>MCGIWALFGSDDCLSVQCLSAMKIAHRGPDAFRFENVNGYTNCCFGFHRLAVVDPLFGMQPIRVKKYPYLWLCYNGEIYNHKKMQQHFEFEYQTKVDGEIILHLYDKGGIEQTICMLDGVFAFVLLDTANKKVFLGRDTYGVRPLFKAMTEDGFLAVCSEAKGLVTLKHSATPFLKVEPFLPGHYEVLDLKPNGKVASVEMVKYHHCRDVPLHALYDNVEKLFPGFEIETVKNNLRILFNNAVKKRLMTDRRIGCLLSGGLDSSLVAATLLKQLKEAQVQYPLQTFAIGMEDSPDLLAARKVADHIGSEHYEVLFNSEEGIQALDEVIF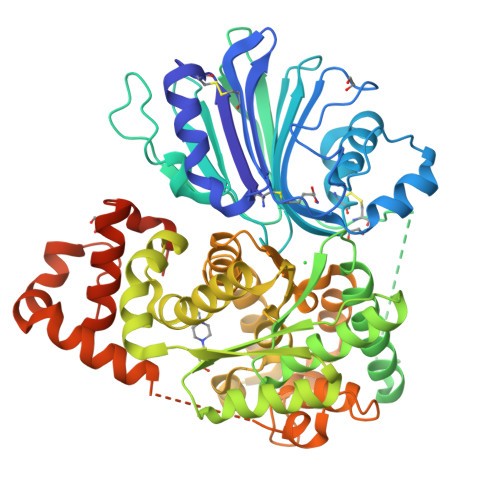SLETYDITTVRASVGMYLISKYIRKNTDSVVIFSGEGSDELTQGYIYFHKAPSPEKAEEESERLLRELYLFDVLRADRTTAAHGLELRVPFLDHRFSSYYLSLPPEMRIPKNGIEKHLLRETFEDSNLIPKEILWRPKEAFSDGITSVKNSWFKILQEYVEHQVDDAMMANAAQKFPFNTPKTKEGYYYRQVFERHYPGRADWLSHYWMPKWINATDPSARTLTHYKSAVKA[2x]> ARVTVQDAVEKIGNRFDLVLVAARRA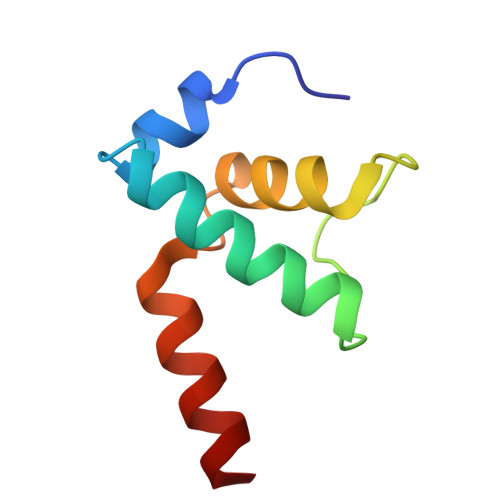RQMQVGGKDPLVPEENDKTTVIALREIEEGLINNQILDVRERQEQQE> EVYGIIAMQAAYRDYDSGDAKQDDNLGGMQLNNESRIGFRGKKQFANFE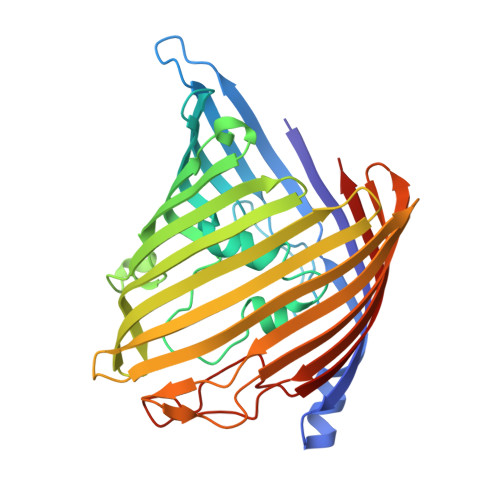PTFIWQIEGGYVDPSFGGEGAGLGERDTFVGFESASWGQVRLGRVLTPMYELVDWPASNPGLGDVYDWGGAIGGAKYQDRQSNTIRWDSPMYADKFSIDAAVGAGDKAGLGAGDDYWGGIAAHYKLGPLQLDAAYEGNRNIEAEGQTWENNTYLVGVQGWFENGISFFAQYKYMEADASNGVNEKQDAMSAGLMYTTGDWQYKLGYAANFDLERDGKTLSNTSDDVVSAQIMYFVDPSAVLYARARMNDFNEGLDGLDDAARWTSGTNGDYNEYSVGVEYYF> CCGCGCCCGUCACACCAC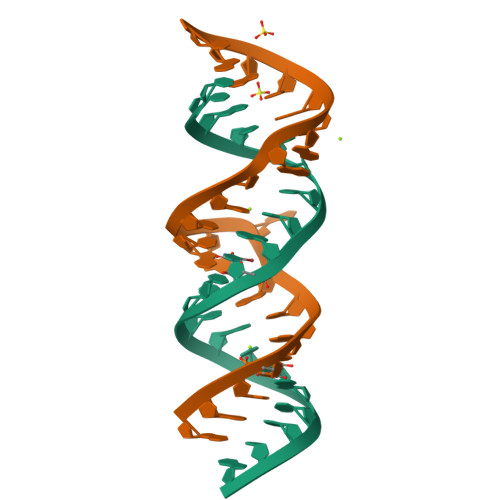CCG;> GGGUGGUGAAGUCGUAACGCGGC Here, we used SthK, a cyclic nucleotide-modulated channel from Spirochaeta thermophila, to define a ligand-gating trajectory that includes multiple on-pathway intermediates. cAMP is a poor partial agonist for SthK and depolarization increases SthK activity. CNG channels are tetrameric channels where each subunit consists of a voltage sensing domain (VSD, S1–S4), a pore domain (S5-S6), and a cytosolic cyclic nucleotide binding domain (CNBD) that is linked to the pore domain via a C-linker comprised of four α helices. Meanwhile, membrane depolarization increases cAMP-induced channel activity, suggesting that voltage modulates the agonist status of cAMP in SthK, similar to its action on other CNG channels, although the mechanism is not known. Cryo-EM structures of VSD mutants with increased activity yielded cAMP-bound closed states (identical to apo and cAMP-bound WT SthK), as well as four additional states: one gating intermediate and 3 open states with different degrees of opening.

Similarly, the sidechain of Arg120, another basic residue on the S4 helix, points into an electronegative pocket formed by Asp61, Ser80, Asp84, and Ser117 on the S2 and S3 helices. Removal of the positive charge of Arg120 would also weaken interactions between S4 and the neighboring helices, facilitating VSD movements in the membrane. We next solved the structures of SthK R120A. Again, as predicted, most of the particles were in a closed conformation (799349 particles, ~76 %), virtually identical to that of WT SthK and SthK Y26F (RMSDs between the closed state structures of each mutant with respect to WT SthK are 0.4 and 0.7 Å, respectively). Again, similar to SthK Y26F, the R120A mutation does not lead to any local or other changes in the channel as gleaned from the identical structures of WT SthK and SthK R120A in the closed state. In all three open conformations of SthK R120A, the lower two helical turns of the S4 helix of the VSD are displaced outwards by a small kink at Val118, allowing S5 to move, which creates space for the expansion of S6. This lateral displacement is not observed in the closed states, which show identical S4 helices in SthK WT, Y26F, and R120A. In both cases, SthK Y26F and SthK R120A, the mutation did not lead to different protein conformations at rest but altered the relative stabilities between closed and open states. Importantly, at 0 mV, the condition on the cryo-EM grid, the extrapolated Po of both mutant channels is ~0.25, more than doubling the activity previously observed for WT SthK (~0.1).

>MAKDIGINSDPNSSSVDKLMKSSGVSNPTYTLVWKVWILAVTLYYAIRIPLTLVFPSLFSPLLPLDILASLALIADIPLDLAFESRRTSGRKPTLLAPSRLPDLLAALPLDLLVFALHLPSPLSLLSLVRLLKLISVQASATRILSYRINPALLRLLSLVGFILLAAHGIACGWMSLQPPSENPAGTRYLSAFYWTITTLTTIGYGDITPSTPTQTVYTIVIELLGAAMYGLVIGNIASLVSKLDAAKLLHRERVERVTAFLSYKRISPELQRRIIEYFDYLWETRRGYEEREVLKELPHPLRLAVAMEIHGDVIEKVPLFKGAGEEFIRDIILHLEPVIYGPGEYIIRAGEMGSDVYFINRGSVEVLSADEKTRYAILSEGQFFGEMALILRAPRTATVRARAFCDLYRLDKETFDRILSRYPEIAAQIQELAVRRKELESSGLVPRGSVKHHHH[4x]>[2x]SEQDCKYWPNCANPLCAFRHPTMPPCRNGGECKVPGCKFTHLKTPCK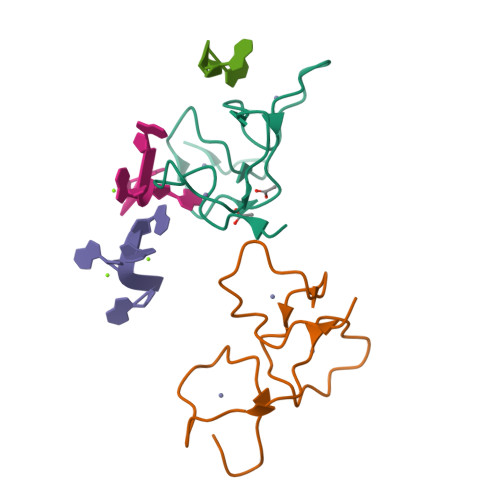FRPCTNRSCPFLHEEGQRG>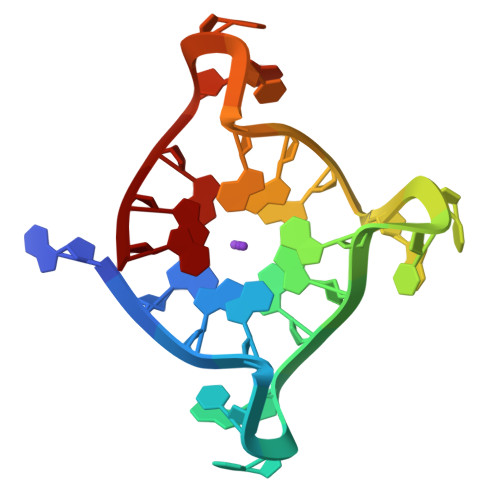 AGGGTTAGGGXTAGGGTTAGGG> 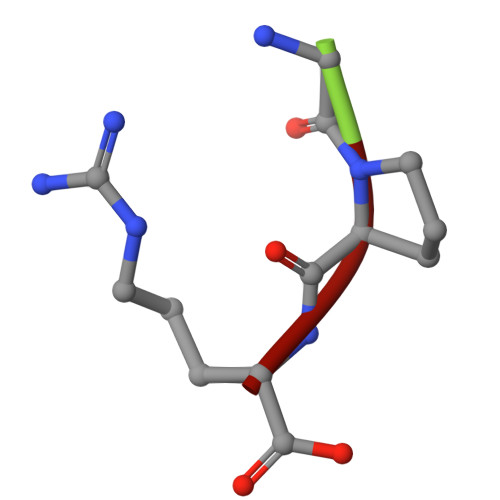GPR> PTHIAICLYYKLGETPLPLVIETG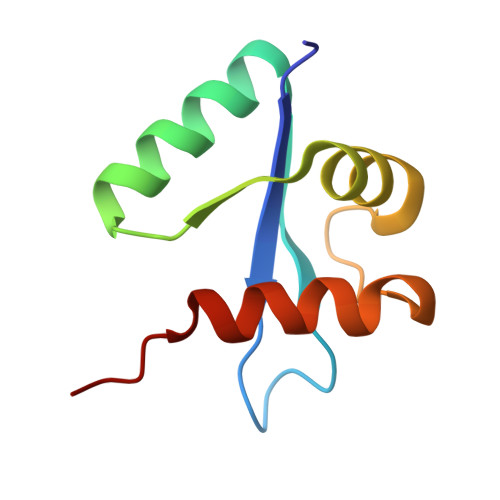KDAKALQIIKLAELYDIPVIEDIPLARSLDKNIHKGQYITEDFFEPVAQLIRIAIDLDY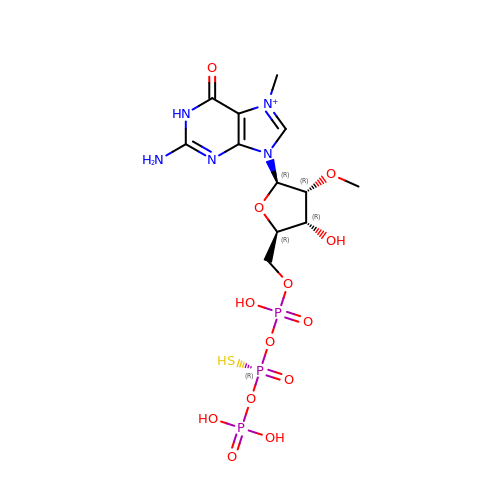[(2~{R},3~{R},4~{R},5~{R})-5-(2-azanyl-7-methyl-6-oxidanylidene-1~{H}-purin-7-ium-9-yl)-4-methoxy-3-oxidanyl-oxolan-2-yl]methyl [phosphonooxy(sulfanyl)phosphoryl] hydrogen phosphate | C12 H21 N5 O13 P3 S | NSORGZXNYGWJBQ-ZRDSBRMSSA-O The resulting UDP-N-acetylglucosamine enolpyruvate (UNAGEP) is reduced by the UNAGEP reductase, MurB, to generate UNAM. All MurB proteins known to date are monomeric flavoenzymes that bind strongly a stoichiometric amount of flavin adenine dinucleotide (FAD). The catalytic cycle can be divided into two half reactions and follows the scheme of a ping-pong bi bi mechanism. Here, we present the crystal structure of NADP+-bound PaMurB, which establishes the co-localization of the NADPH and UNAGEP binding sites and supports a ping pong reaction mechanism with sequential substrate binding.

Crystal form A belongs to the space group C2 with four molecules per asymmetric unit, while crystal form B belongs to P61 with one molecule per asymmetric unit; the solutions are in agreement with solvent content analysis by using Matthews coefficient. Also for crystal form A, the resulting electron density maps were of good quality, most likely due to the presence of four-fold non-crystallographic symmetry. A strong residual electron density in the vicinity of the nicotinamide ring was modeled as a metal ion in crystal form A. Refinement with potassium gave the most satisfactory results in terms of B factors and difference densities. The metal site is located at the active site in the vicinity of the nicotinamide and the isoalloxazine rings of NADP+ and FAD, respectively. The potassium ion displays a pentagonal bipyramidal coordination geometry with two main chain oxygen atoms (Ala-237, Ser-239), one side chain carboxyl oxygen atom from Glu-335, one side chain oxygen atom of Asn-57 and the O7n oxygen atom of the nicotinamide ring as ligands. The interactions between Glu-335, nicotinamide and the metal ion position the nicotinamide C4n 3.1 Å from the isoalloxazine N5, and 109.3° from the isoalloxazine plane (defined as the C4n-N5-N10 angle). Potassium binding apparent in only crystal form A could be due to the five times higher potassium concentration in the crystallization liquor for form A compared to form B crystals. It is noteworthy that the potassium concentration used to grow crystal form A is closer to physiological concentrations of this metal ion in the bacterial cell than the significantly lower concentration in form B crystals. The observation of a bound potassium ion in the crystal structure of PaMurB provides a structural and chemical explanation for these findings.

>SMSLELQEHCSLKPYNTFGIDVRARLLAHARDEADVREALALARERGLPLLVIGGGSNLLLTRDVEALVLRMASQGRRIVSDAADSVLVEAEAGEAWDPFVQWSLERGLAGLENLSLIPGTVGAAPMQNIGAYGVELKDVFDSLTALDRQDGTLREFDRQACRFGYRDSLFKQEPDRWLILRVRLRLTRRERLHLDYGPVRQRLEEEGIASPTARDVSRVICAIRREKLPDPAVLGNAGSFFKNPLVDATQAERLRQAFPDLVGYPQADGRLKLAAGWLIDKGGWKGFRDGPVGVHAQQALVLVNHGGATGAQVRALAERIQEDVRRRFGVELEPEPNLY[4x]> MKILLIGMGGTIASVKGENGYEASLSVKEVLDIAGIKDCEDCDFLDLKNVDSTLIQPEDWVDLAETLYKNVKKYDGIIVTHGTDTLAYTSSMISFMLRNPPIPIVFTGSMIPATEENSDAPLNLQTAIKFATSGIRGVYVAFNGKVMLGVRTSKVRTMSRDAFESINYPIIAELRGED;> MAVLVIKLIPGLSGDIFRAAVELGYRGIVIEGYGAGGIPYRGSDLLQTIEELSKEIPIVMTTQAMYDGVDLTRYKVGRLALRAGVIPAGDMTKEATVTKLMWILGHTNNVEEIKVLMRKNLVGELRD;>LVVN[2x]

Variable temperature solution light scattering and/or SAXS experiments have provided important findings about influence of temperature on protein shape or association levels which expand our understanding. Previously, we provided a detailed structural and mechanistic insight of thermophilic l-asparaginase from Pyrococcus furiosus in its full-length (PfA), and a conjoined functional version (cPfA) (domain architecture shown in Supplementary Fig. S1). SAXS and crystal diffraction data analysis brought forth that despite lacking a 19-residue long linker which connects the two domains, namely the N- and C-halves (N-PfA and C-PfA, respectively), cPfA adopts a solution shape and crystalline state that is comparable to wild type full-length protein PfA with improved specific-activity. In conclusion, the findings reported here provide structural evidence in support of temperature induced higher order oligomer formation conferring stability to thermophilic proteins thereby regulating their functioning.

To further investigate if the terminal β-strand of the N-terminal domain is important in providing stability through oligomerization under high temperature conditions, we truncated cPfA beyond D178 and named it as defunct cPfA (dcPfA). Our crystallization attempts of dcPfA were unsuccessful. Diffraction data was collected up to 2.61 Å resolution. wo additional electron densities were observed in both fo − fc and 2fo − fc maps. One of the electron densities was present at the same site where residues were truncated from cPfA (named e’ density 1) while the second was present near the residues 42–45 (named e′ density 2). The results showed residue E173 of dcPfA was interacting with V2 of peptide (corresponding protein residue is V180) through two H-bonds. Thus, as all the interactions between P1 and dcPfA were identical to those present in cPfA, the peptide successfully restored the structural features of parent protein. Later on, successful crystallization of dcPfA with LVVN peptide where latter retains its location at the speculated site (where the terminal β-strand was originally present in the parent protein) re-established the structural stability and thus also restored functionality. At the highest effective peptide concentration i.e. 500 µM, the specific activity increased by 1.66-fold, 1.85-fold and 2.36-fold at 37 °C, 45 °C and 60 °C, respectively, as compared to dcPfA alone. Such peptide-mediated activity restoration depicted that the peptide probably binds the same sites where these residues were intact originally in cPfA (supported from dcPfA-peptide bound crystal structure data, Fig. 4B), thereby reconciling interactions between native functional assemblies.>IDGFVRTLRARPEAGGKVPVFVFHPAGGSTVVYEPLLGRLPADTPMYGFERVEGSIEERAQQYVPKLIEMQGDGPYV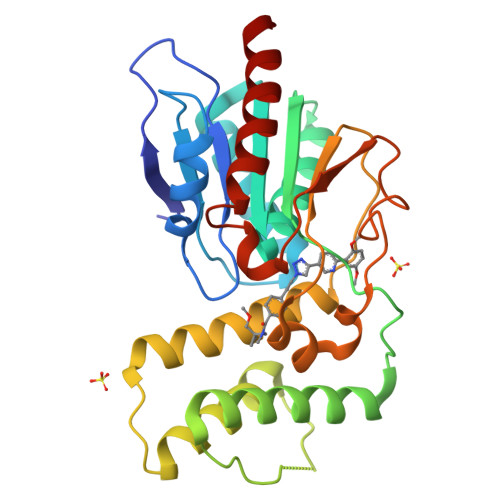LVGWSLGGVLAYACAIGLRRLGKDVRFVGLIDAVRAGEEIPQTKEEIRKRWDRYAAFAEKTFNVTIPAIPYEQLEELDDEGQVRFVLDAVSQSGVQIPAGIIEHQRTSYLDNRAIDTAQIQPYDGHVTLYMADRYHDDAIMFEPRYAVRQPDGGWGEYVSDLEVVPIGGEHIQAIDEPIIAKVGEHMSRALGQIEADR[2x]4-{[(1R)-6-methoxy-1-methyl-1-{2-oxo-2-[(1,3-thiazol-2-yl)amino]ethyl}-1,2,3,4-tetrahydroisoquinolin-7-yl]oxy}benzoic 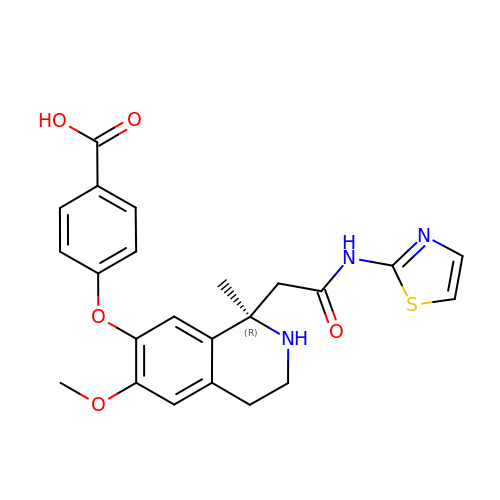acid | C23 H23 N3 O5 S | CPPVZZXHKAJGRZ-HSZRJFAPSA-N> SNSLHWPTSLPSGDAFSSVGTHRFVQKVEEMVQNHMTYSLQDVGGDANWQLVVEEGEMKVYRREVEENGIVLDPLKATHAVKGVTGHEVCNYFWNVDVRNDWETTIENFHVVETLADNAIIIYQTHKRVWPASQRDVLYLSVIRKIPALTENDPETWIV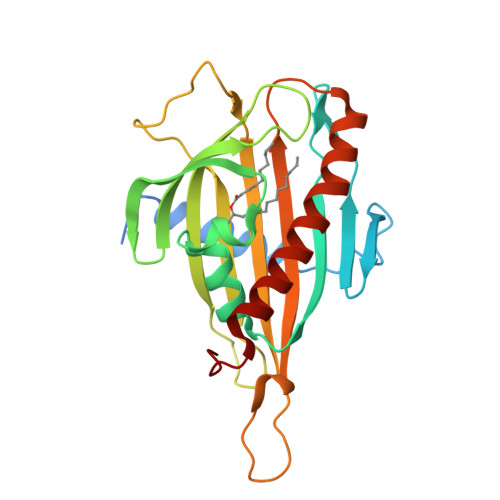CAFSVDHDSAPLNNRCVRAKINVAMICQTLVSPPEGNQEISRDNILCKITYVANVNPGGWAPASVLRAVAKREYPKFLKRFTSYVQEKTAGKPILF> SSFSQHARTSGRVAVEEVDEEGKFVRLRNKSNEDQSMGNWQIKRQNGDDPLLTYRFP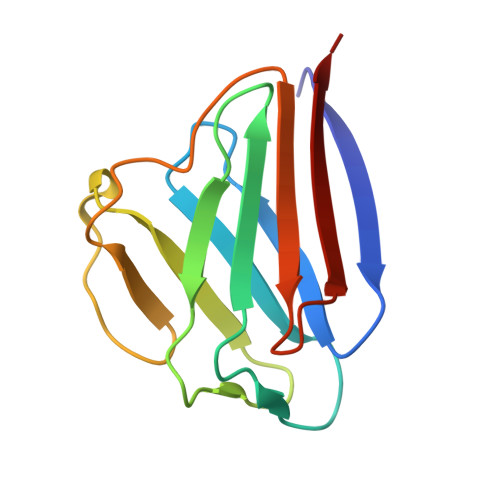PKFTLKAGQVVTIWAAGAGATHSPPTDLVWKAQNTWGCGNSLRTALINSTGEEVAMRKLVRS> SLRECELYVQKHNIQALLKDSIV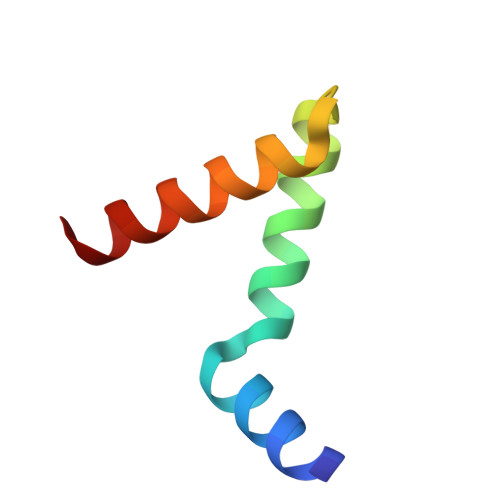QLCTARPERPMAFLREYFEKLEKEEAK>GHMGQKASQQLALKDSKEVPVVCEVVSEAIVHAAQKLKEYLGFEYPPSKLCPAANTLNEIFLIHFITFCQEKGVDEWLTTTKMTKHQAFLFGADWIWTFWGSDKQIKLQLAVQTLQMSSPPPVESKPCDLSNPESRVEESSWKKSRFDKLEEFCNLIGEDCLGLFIIFGMPGKPKDIRGVVLDSVKSQMVRSHLPGGKAVAQFVLETEDCVFIKELLRNCLSKKDGLREVGKVYISIL[2x];>GHMASVTDGKTGVKDASDQNFDYMFKLLIIGNS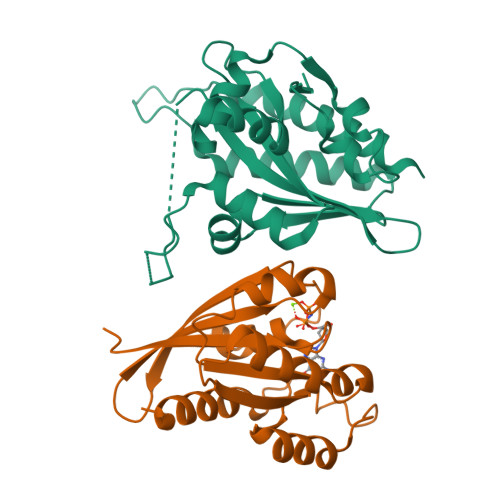SVGKTSFLFRYADDTFTPAFVSTVGIDFKVKTVYRHEKRVKLQIWDTAGQERYRTITTAYYRGAMGFILMYDITNEESFNAVQDWATQIKTYSWDNAQVILVGNKCDMEEERVVPTEKGQLLAEQLGFDFFEASAKENISVRQAFERLVDAICDKMSDSLDTDPSMLGSSKNTRLSDTPPLLQQNCSC[2x]>GSHMEVTEEDIAEIVSRWTGIPVSKLLEGEREKLLRLEEELHKRVVGQDEAIRAVADAIRRARAGLKDPNRPIGSFLFLGPTGVGQTELAKTLAATLFDTEEAMIRIDMTEYMEKHAVSRLIGAPPGYVGYEEGGQLTEAVRRRPYSVILFDEIEKAHPDVFNILLQILDDGRLTDSHGRTVDFRNTVIILTSNLGSPLILEGLQKGWPYERIRDEVFKVLQQHFRPEFLNRLDEIVVFRPLTKEQIRQIVEIQLSYLRARLAEKRISLELTEAAKDFLAERGYDPVFGARPLRRVIQRELETPLAQKILAGEVKEGDRVQVDVGPAGLVFAVPARVEA[3x]

The molecular chaperone ClpB, the bacterial homologue of Hsp104, is a disaggregation machine that provides thermotolerance by resolubilizing and reactivating aggregated proteins in concert with the DnaK (Hsp70) chaperone system. ClpB belongs to the family of AAA+ proteins (ATPases associated with various cellular activities) that comprises a wide range of molecular machines which utilize the energy from ATP hydrolysis to remodel their respective substrates. The AAA+ disaggregation machines Hsp104 and ClpB possess two NBDs per monomer, thus forming double-ring structures with 12 potential ATPase sites in the active hexameric complex. We determined high-resolution X-ray structures in different nucleotide states for one of the motor subunits, namely NBD2, of ClpB and combined the structural analysis with nucleotide-binding kinetics studies.

In order to perturb the open, inactive arrangement of the ClpB NBD2 catalytic site, we replaced the Walker A lysine with a glutamine. To crystallize the mutant ClpB variant NBD2 K601Q, we supplemented the crystallization cocktail with the fluorescently labelled nucleotide MANT-dADP, which has been routinely used for nucleotide-binding studies of ClpB and is known to bind more than 100-fold more strongly to NBD2 than unlabelled ADP. This compensated for the loss in binding affinity owing to the Walker A mutation and allowed us to obtain a nucleotide-bound structure of ClpB NBD2 K601Q. The complex of ClpB NBD2 K601Q and MANT-dADP crystallized from a condition containing PEG 6000 and yielded a different crystal form to that observed previously for the wild-type protein in conditions containing 2-propanol (P212121 instead of P65). The structure was determined by molecular replacement to a resolution of 2.8 Å, showing well defined electron density for the previously unstructured pore-loop region (residues 640–650). The fluorescently labelled MANT-dADP binds at the same position as the unlabelled nucleotides in the structures obtained previously. A domain-motion analysis using DynDom comparing the MANT-dADP-bound form with the ADP-bound form showed that the angle between the domains decreases by 14°. The essential sensor 2 residue Arg806 located on the C-­terminal small domain forms a salt bridge (d = 2.8 Å) with the β-phosphate of the nucleotide. An additional phosphate ion is present in the active site at a distance of 5 Å from the β-­phosphate of the nucleotide, suggesting that we may have captured an ADP + Pi (product-bound) state here. Interestingly, another highly conserved active-site residue, Arg621, adopts a different conformation to that in the structures described previously.Inoviruses are filamentous phages infecting numerous prokaryotic phyla. The first inovirus identified, named fd, was reported in 1963 as a DNA-containing phage with an unusual filamentous morphology infecting Escherichia coli. Fd has since become a model for filamentous phage structure, infection, and assembly, as well as having found use in numerous biotechnological applications, including the first described instance of phage display, and as a model for examining colloidal-rod phase transitions. A unique property of inoviral phages, including fd and Pf4, is that they can spontaneously and reversibly self-assemble to form ordered but dynamic structures termed tactoids under crowding conditions.

Using helical reconstruction and applying C5 symmetry, a 3.2 Å-resolution map of the fd phage capsid was obtained, which allowed derivation of an atomic model of the capsid. In agreement with previous predictions, the atomic model reveals a pentameric (C5) subunit arrangement of the pVIII capsid protein, which forms a single α-helix containing 50 residues. The helix is terminated at the N-terminus of the mature protein by a proline residue (P6), and residues 1–5 of the capsid protein, which are located on the phage surface, are disordered. Due to helical symmetry, capsid protein monomers stack almost vertically to form a highly symmetrical arrangement along the helical axis. The C-terminus of the capsid protein, which faces the inner lumen of the cylindrical phage, interacting with the genomic DNA, has four positively charged lysine residues exposed to the lumen. These lysines presumably bind to the negatively-charged DNA phosphates, as also seen in other phages. While density for the DNA is observed in our fd cryo-EM map, it is not well-resolved and does not support atomic model building of the DNA genome. Our structure suggests that while Y21 is involved in hydrophobic interactions within the capsid, it does not act as a structural hinge, evidenced by our high-resolution map. Structural comparison with Pf44, a class II inoviral bacteriophage with a prophage lifestyle, shows a slightly larger capsid size (fd: 50 residues, Pf4: 46 residues) and lumen diameter (fd: 24 Å, Pf4: 22 Å). In agreement with previous work, our structural model for fd suggests a circular single-stranded arrangement, as the higher positive charge-density of the capsid protein (four basic residues in fd versus two in Pf4) suggests that twice as many negative charges of the DNA phosphate backbone are being stabilised.

> AEGDDPAKAAFDSLQASATEYIGYAWAMVVVIVGATIGIKLFKKFTSKAS>[5x]GAMEMRLEKDRFSVNLDVKHFSPEELKVKVLGDVIEVHGKHEERQDEHGFIS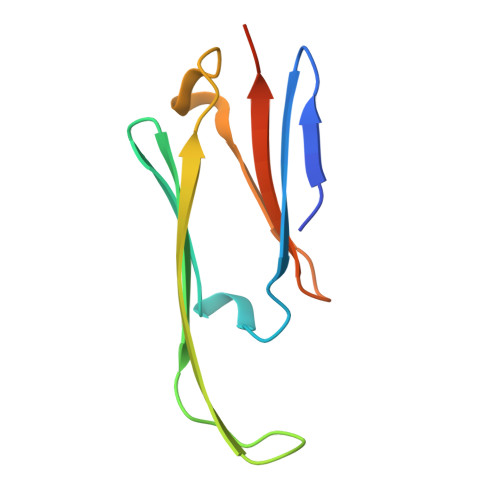REFHRKYRIPADVDPLTITSSLSSDGVLTVNGPRKQVSGPER> SNAMLYPVLTQSRLLSDLSGVWNFKLDNGKGFEEKWYEKPLKDADTMPVPASYNDLKEGTDFRDHYGWVFYQRNISVPEYVKSQRIVLRCAAVTHYAMIYLNGKLICEHKGGFLPFEVELNDDLQDGDNLLTIAVNNVIDYTTLPVGGKANMMSGMMGGMGAGASDKPQNNPNFDFFNYCGITRPVKIYTTPETYINDITVTADIDFTKEEPSAVLNYNVEIKGKDYNNITCKVELFDEEGTKLSETEGSEGTFEISNVRLWQPLNAYLYKIKVTAGQDVYTLPYGVRSVRVDGTKFLINEKPFYFKGYGKHEDTFPNGRGINLPMNTKDISIMKWQHANSFRTSHYPYSEEMMRLCDEEGIVVIDETTAVGVNLQFGGGANFGGERIGTFDKEHGVQTQEHHKDVIRDLISRDKNHACVVMWSIANEPDSAAEGAYDYFKPLYDLA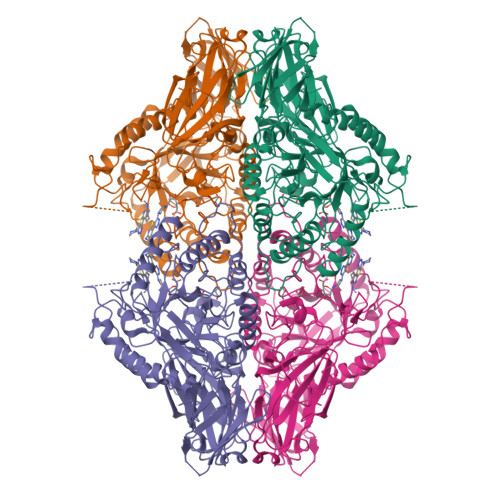RELDPQKRPCTLVSVQGTTADTDCSSQLSDVICLNRYYGWYFGGPDLEVSETGLRKELSDWGKLGKPVMFTEYGADTVSGLHDTTSVMYTEEYQVEYYEMNNKVFDEFDFVVGEQAWNFADFATSQSLLRVQGNKKGLFTRDRKPKMVAHYFRNRWSAIPEFGYKTK> MARQNS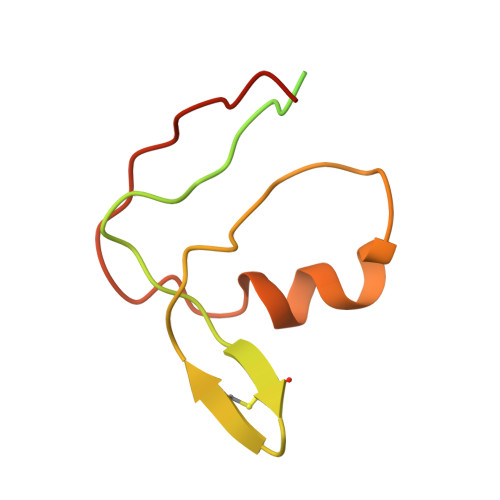AAKTTAKSKTDPATEKPKDDTLPDSTDDASPTAPETPATKPDSASDEVEGVFVRATVERRCRAGFCFDKEGQGFADGVLSDEQLEALESDPLLKVERCTFSGNQEGE> MTARIALASLFVVAAVLAQPWQTTTQRWVLGVSIAAVIVLLAWWKGMFLTTRIGRALAMVRRNRAEDTVETDAHRATVVL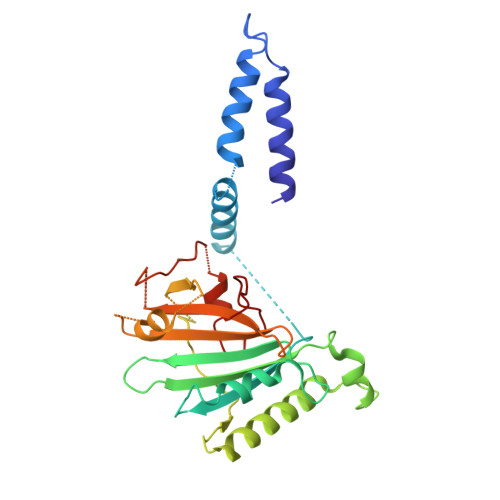RVDPAAPAQLPVVVGYLDRYGITCDKVRITHRDAGGTRRSWISLTVDAVDNLAALQARSARIPLQDTTEVVGRRLADHLREQGWTVTVVEGVDTPLPVSGKETWRGVADDAGVVAAYRVKVDDRLDEVLAEIGHLPAEETWTALEFTGSPAEPLLTVCAAVRTSDRPAAKAPLAGLTPARGRHRPALAALNPLSTERLDGTAVPL> TSFXEYWAL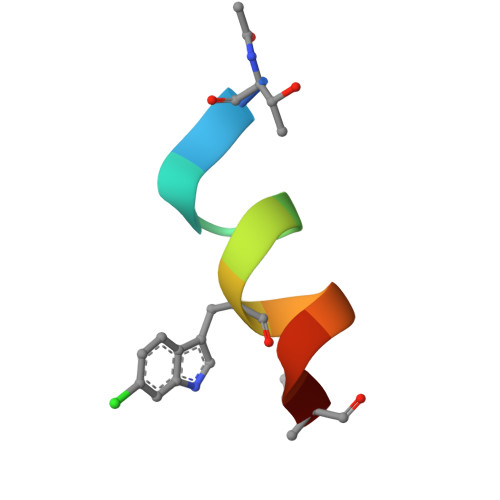LLX During the initiation step of bacterial genome replication, replicative helicases depend on specialized proteins for their loading onto oriC. The toroidal hexameric helicase DnaB is then loaded onto the locally open DNA duplex, with the help of a helicase loader, triggering the recruitment of the various proteins of the replisome. However, most bacteria do not contain any of these genes, which are domesticated phage elements that have replaced the ancestral and unrelated loader gene dciA several times during evolution. Through multiple complementary approaches, we previously established that the disordered CTD of DciA can form transiently small helical structures and is necessary for interacting with DnaB and stimulating the loading of DnaB onto DNA.

To decipher the molecular interactions between DciA and DnaB, we solved the crystal structure of the DnaB·DciA complex from Vibrio cholerae (Vc) together with ADP and Mg2+, forming a heterotetramer composed of the canonical VcDnaB dimer and two molecules of VcDciA. The asymmetric unit of the crystal contains two molecules of VcDnaB and two molecules of VcDciA. The crystal structure of the VcDnaB·VcDciA complex revealed domain swapping between symmetry-related molecules of VcDciA. The NTD and CTD (N-terminal and C-terminal domains) of two VcDciA molecules connected by an extended hinge region (residues Glu99–Ser121) are exchanged between neighboring molecules related by a true crystallographic twofold rotation axis. Therefore, formation of the complex with VcDciA does not alter the overall canonical architecture of the VcDnaB dimer or the NTP binding site. Interestingly, the CTD tail of VcDciA, which was observed to be disordered in solution by SAXS, folds into a small helix hairpin in contact with VcDnaB, again in agreement with our previous molecular-dynamics analyses.

>[2x]MADPRTDNRNRKIPDAQVDAIKVPPHSLEAEQSVIGGLLLDNERWDTVSEHVMTQDFYSRPHRLIFDGVKSILEAGKPLDLITLSEYLEQREQLEDVGGFAYLADLAKNTPSAANINAYAEIVAERALVRNLIGVANEIADAGYDPQGRNAEDLLDLAESKVFAIAEARTSENEGPKNVDSILERTLERIELLYKTPQDGVTGVNTGFTDLNKKTAGLQGSDLIIVAARPSMGKTTFAMNLCENAAMEQDKPVLIFSLEMPAEQIMMRMLASLSRVDQTKIRTGQLDDEDWARISSTMGILMEKKNMYIDDSSGLTPTEVRSRARRIAREHGGLSLIMVDYLQLMRVPALTDNRTLEIAEISRSLKALAKELNVPVVALSQLNRSLEQRADKRPVNSDLRESGSIEQDADLIMFIYRDEVYHPDSPLKGTAEIIIGKQRNGPIGSVRLTFQGHYSRFDNYAGPAFDDEHHHHHH;>[2x]MHHHHHHRDHRPTATDELIQASKLKQIQEHAKAILLINRQLQDILPKGLKTQVRAANVRGGNLVLEAASAALKMKVDYERLHILTQLRQNGFGHLISIEVRVNPELYRQSKITSEDARAANPRPPLSEHAAHVLLAIADQASDKVKKRLQSLARLAKANQKDD> SNAMADEIAKAQVARPGGDTIFGKIIRKEIPAKIIFEDDRCLAFHDISPQAPTHFLVIPKKHISQISVAEDDDE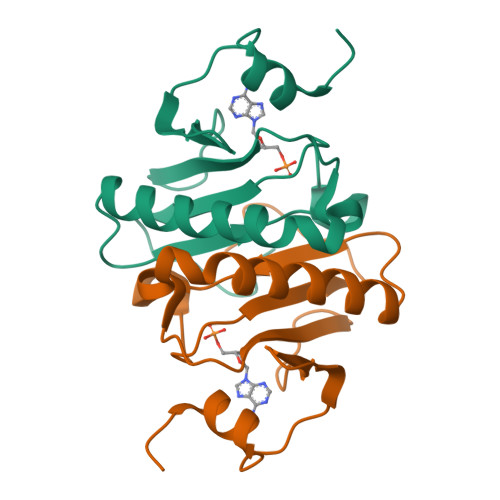SLLGHLMIVGKKCAADLGLNKGYRMVVNEGSDGGQSVYHVHLHVLGGRQMHWPPG> KTPADNIETADLSASVPTRPAEPERKTLADYGGYPSALDAVKQKNDAAVAAYLENAGDSAMAENVRNEWLKSLGARRQWTLFAQEYAKLEPAGRAQEVECYADSSRNDYTRAAELVKNTGKLPSGCTKLLEQAAASGLLDGNDAWRRVRGLLAGRQTTDARNLAAALGSPFDGGTQGSREYALLNVIGKEARKSPNAAALLSEMESGLSLEQRSFAWGVLGHYQSQNLNVPAALDYYGKVADRRQLTDDQIEWYARAALRARRWDELASVISHMPEKLQKSPTWLYWLARSRAATGNTQEAEKLYKQAAATGRNFYAVLAGEELGRKIDTRNNVPDAGKNSVRRMAEDGAVKRALVLFQNSQSAGDAKMRRQAQAEWRFATRGFDEDKLLTAAQTAFDHGFYDMAVNSAERTDRKLNYTLRYISPFKDTVIRHAQNVNVDPAWVYGLIRQESRFVIGAQSRVGAQGLMQVMPATAREIAGKIGMDAAQLYTADGNIRMGTWYMADTKRRLQNNEVLATAGYNAGPGRARRWQ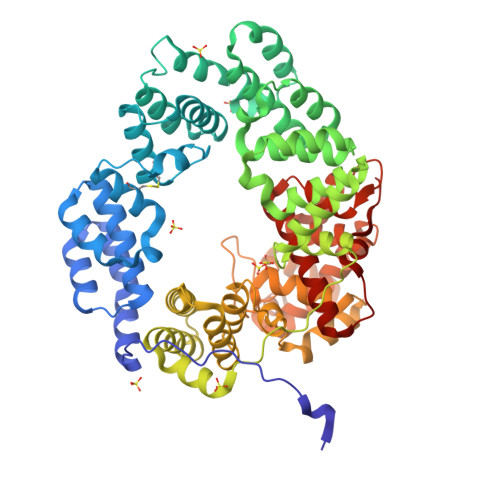ADTPLEGAVYAETIPFSETRDYVKKVMANAAYYAALFGAPHIPLKQRMGIVPAR>[2x]MAEKLHISVLCGGQSTEHEISIQSAKNIVNTLDAAKYLISV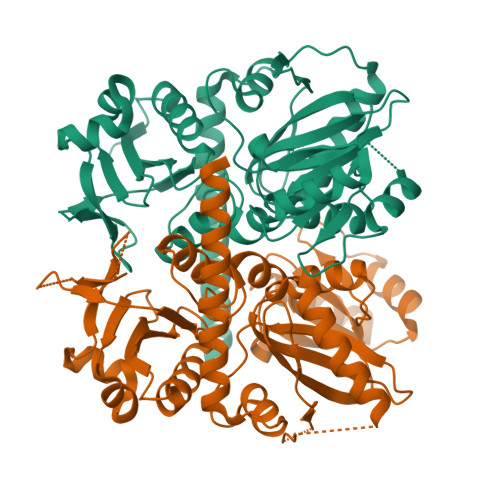IFIDHVGRWYLIDQPEMFLAHSPDHLVKEGSARPITIAFGDAAKPWQSLNGDGRRYSADCVFPMVHGTQGEDGALQGLLELLNLPYVGANVQSSAVCMEKDLTKTVLRAGGIPVVDWHTLSPRDATEGVYQRLLDRWGTSELFVKAVSLGSSVATLPVKTETEFTKAVKEVFRYDDRLMVEPRIRGREIECAVLGNGAPKASLPGEIIPHHDYYSYDAKYLDPNGATTTTSVDLSESVTKQIQQIAIDAFKMVHCSGMARVDFFVTPNNKVLVNEINTIPGFTNISMYPKMWEASGLPCPNLLDQLIELAIDRHQEQQKLIRCYEVKARSL>GADDELYRQSLEIISRYLREQATGAKDTKPMGRSGATSRKALETLRRVGDGVQRNHETAFQGMLRK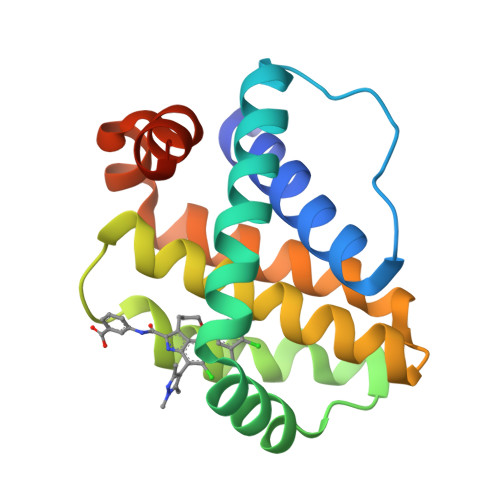LDIKNEDDVKSLSRVMIHVFSDGVTNWGRIVTLISFGAFVAKHLKTINQESCIEPLAESITDVLVRTKRDWLVKQRGWDGFVEFFHVEDLEGG[4x]7-({[3-(5-fluoropyridin-3-yl)propyl]amino}methyl)quinolin-2-amine | C18 H19 F N4 | 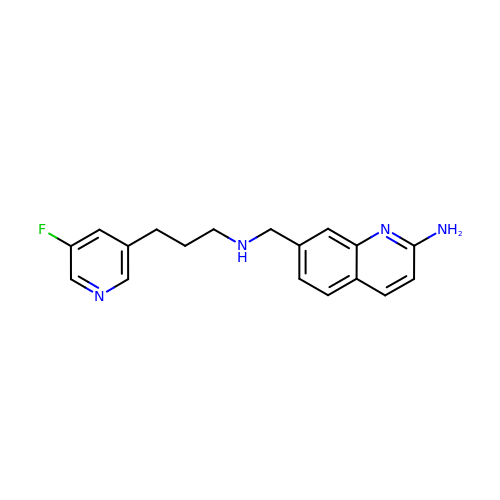GIUCGMWNASMMOJ-UHFFFAOYSA-N> GSTAEKDKLPATQKAKEMQNVPYTIAVDGIMAFNQSYLNLPKDSQLSYLDLGNKVKALLYDERGVTPEKIRNAKSAVYTITWKDGSKK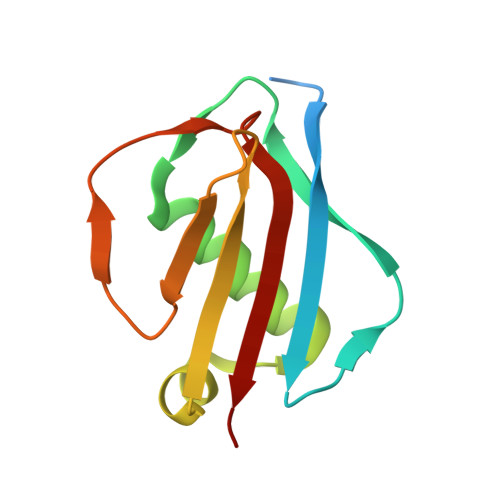EVDLKKDSYTANLFDSNSIKQIDINVKTK> GHMGIQHEFDIIINGDIALRNLQLHKGDNYGCKLKIISNDYKKLKFRFIIRPDWSEIDEVKGLTVFANNYAVKVNKVDDTFYYV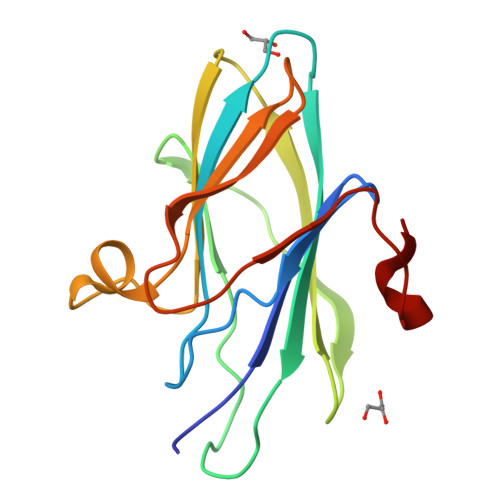IYEAVIHLYNKKTEILIYSDDENELFKHYYPYISLNMISKKYKVKEENYSSPYIEHPLIPYRDYESMD> MAINKNKVITKKQTIPAFFKGNAPYIFAHRGGM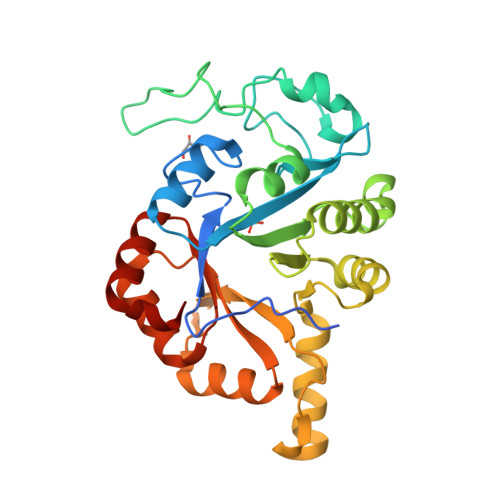ALRPEQTQLAFDYAKQLGVDGFETDVRLTKDQQLIVFHDATVDRTTNGSGKVSAHTLAELKKLDAAYHFKDINGLTPYRGHAHTAILTFDELLKQYPDMYINVDLKDAPESYEGSIAPQIMFDTIAENQAFDRVLVTSFYKEQIVRFNKIAQGSVAIGASQQEVTEAFLKYHLLGGRYYQPLAQTFQMPTHFKGIDLTSSRFIKWLNDMNIIPGYYGVNSINLMNDLYQKGAHTIVTDRPDLAQQFKQTIPNKLEHHHHHH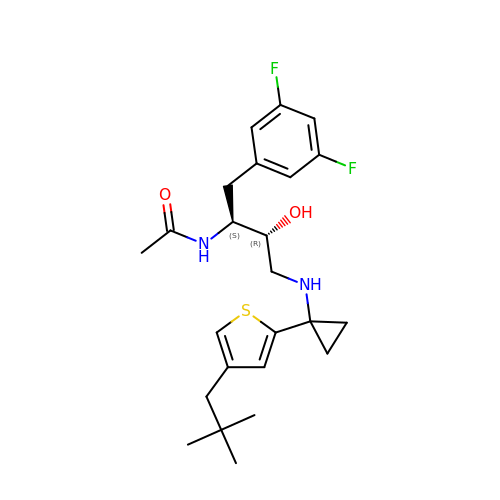N-[(1S,2R)-1-(3,5-difluorobenzyl)-3-({1-[4-(2,2-dimethylpropyl)thiophen-2-yl]cyclopropyl}amino)-2-hydroxypropyl]acetamide | C24 H32 F2 N2 O2 S | YEGCCSKZPHGALE-LEWJYISDSA-N> APRGTHL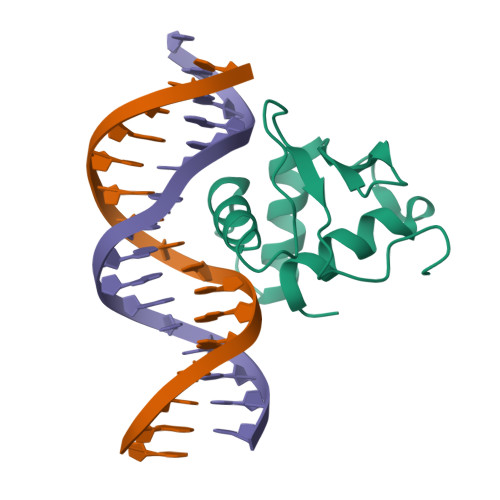WEFIRDILIHPELNEGLMKWENRHEGVFKFLRSEAVAQLWGQKKKNSNMTYEKLSRAMRYYYKREILERVDGRRLVYKFGKNSSGWKEEEVGESRN> RG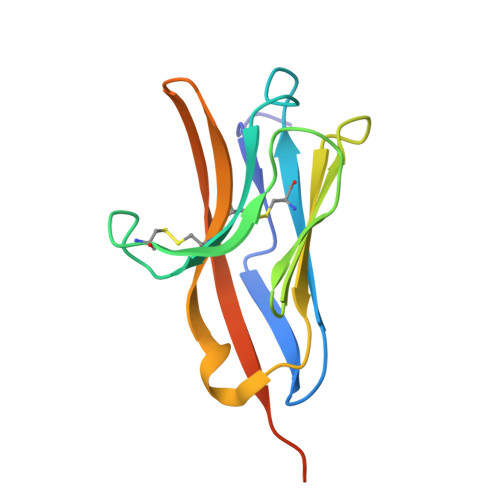IPQITGPTTVNGLERGSLTVQCVYRSGWETYLKWWCRGAIWRDCKILVKTSGSEQEVKRDRVSIKDNQKNRTFTVTMEDLMKTDADTYWCGIEKTGNDLGVTVQVTIDPAPVTQEETSSSPT> MDLAYVCEWEKWAKSTYCPSLPLACAWSCRNLIAFTTDLRNDDQDLTHMIHILDTEHPWEVHSVSSGHSEAITCLEWDQSGSRLLSADADGQIKCWSMADHLANSWESSVGSQVEGDPIVALSWLHNGVKLALHVEKSGASSFGEKFSRVKFSPSLTLFGGKPMEGWIAVTVSGLVTVSLLKPSGQVLTSTESLCRLRGRVALADIAFTGGGNIVVAAADGSSASPVKFYKVCVSVVSEKCRIDTEILPSLFMRCTTDPNRKDRFPAITHLKFLARDMSEQVLLCASSQTSSLVECWSLRKEGLPVNNIFQQISPVVGDKQPMILKWRILSATNDLDRVSAVALPKLPISLTNTDLKVASDTQFYPGLGLALAFQDGSVHMVHRLSLQTMAVFYSSAPRSLDEPALKRPRTTCPAVHFKAMQLSWTSLALVGIDNHGKLSMLRISPSLGHPLEPKLALQHLLFLLEYCMVTGYDWWDILLHVQPGMVQSLVERLHEEYTRQKPALQQVLSTRILAMKASLCKLSPCTVARVCDYHTKLFLMAIT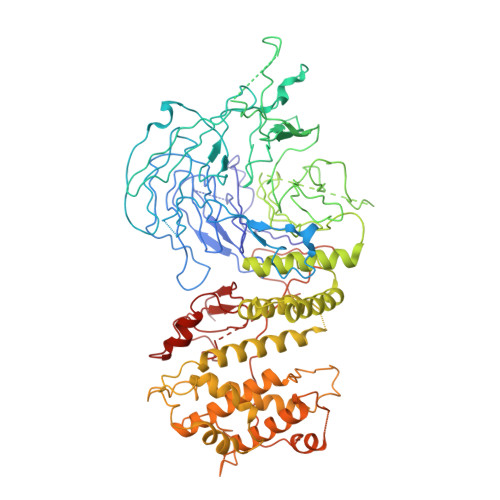STLKSLLRPHFLNTPDKSPGDRLAEICAKITDVDIDKVMINLKTEEFVLDMNTLQALQQLLQWVGDFVLYLLVSLPNQGSPLRPGHSFLRDGTSLGMLRELMVVIRIWGLLKPSCLPVYTATSDTQDSMSLLFRLLTKLWICCRDEGAASEPDEGLVDECCLLPSQLLVPNLDWLPASDGLVSRLQPKQPLRLRFGRAPTLPSSTSTLQLDGLTRAPGQPKIDHLRRLHLGAYPTEECKACTRCGCVTMLKSPNKTTAVTQWEQRWIKNCLCGGLWRRVPLSCS>MAEYVFSDAPKDSHGNGVKDAVPGKQPEELPPAPRYFQGENTAGFMRPVRFEGDITNLEVVGEIPKSIEGTFYRVMPEPHLPSFIPNDPWFNGDGNISGFYFKDGHVDLKQRYVRTEKFVREAEARRSLLGKYRNRYTDLVEFKIRSTANTNIVYWRGQLLALKEDSPPYAMDPETLETFGVYDFDGQLPSLTFTAHPKFDPVTREMVCFGYEAKGDGTRDICYYSFGPDGKIAETVWLVSPVCGMIHDFAVTENFVIFPIIPLVCDVERMKQGGDHWQWDYSIPMYIGVLPRRGAQGSDVKWFEAPHGFAGHVANAFEDDKGHIQLQMAYAKDNVFFWWPDANGKGPRPGEVEAHFANFVLDYQSDKLPLAEPTYLVDDDMEFPRIDDRVATRKHKHTFFCIFDRKPGVTDFEFVMPRAGGGAPMSNGLAHLNHETGDIQRYLPGPRKLTGECIFIPRNSEAAEGDGYVMVLLANYEDMCSELAVLDTKDLTNEVALIKLPVRLRPGLHGNWVDKSDVDGHPAP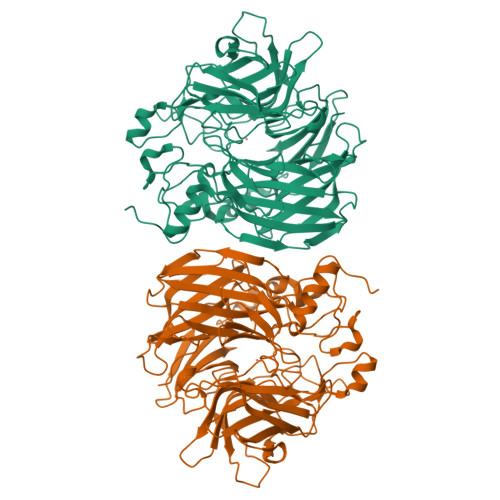L[4x]> MHTAEFLETEPTEISSVLAGGYNHPLLRQWQSERQLTKNMLIFPLFISDNPDDFTEIDSLPNINRIGVNRLKDYLKPLVAKGLRSVILFGVPLIPGTKDPVGTAADDPAGPVIQGIKFIREYFPELYIICDVCLCEYTSHGHCGVLYDDGTINRERSVSRLAAVAVNYAKAGAHCVAPSDMIDGRIRDIKRGLINANLAHKTFVLSYAAKFSGNLYGPFRDAACSAPSNGDRKCYQLPPAGRGLARRALERDMSEGADGIIVKPSTFYLDIMRDASEICKDLPICAYHVSGEYAMLHAAAEKGVVDLKTIAFESHQGFLRAGARLIITYLAP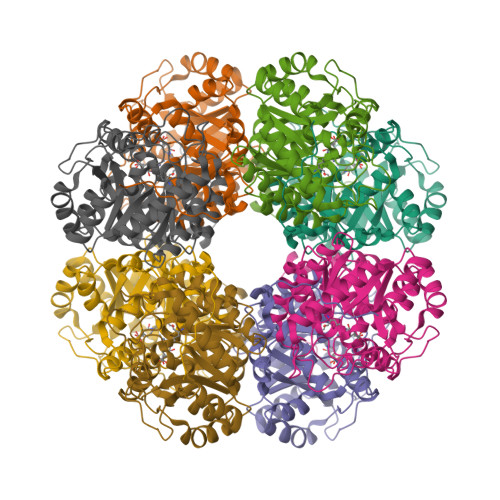EFLDWLDEEN> QDYGGFPAPILRAVPSAEPQAGSPMTLSCQTKLPLQRSAARLLFSFYKDGRIVQSRGLSSEFQIPTASEDHSGSYW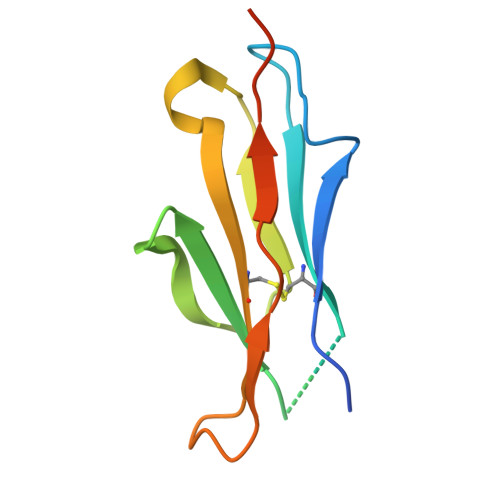CEAATEDNQVWKQSPQLEIRVQGASAENLYFQ(2~{S})-2-acetamido-~{N}-(3-bromanylpropyl)-3-methyl-butanamide | C10 H19 Br N2 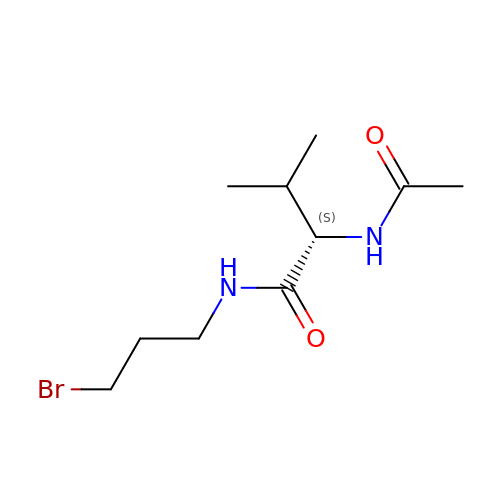O2 | IEVYCEWEWALKSB-VIFPVBQESA-N> CC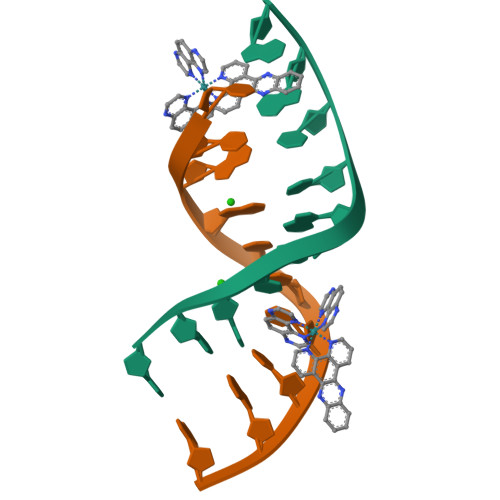GGCTCCGG;> CCGGAGCCGG>SNLEQIDAELVLSIEKLQEIQDDLEKINEKASDEVLEVEQKYNVIRKPVYDKRNEVIQSIPGFWMTAFLSHPALGDLLTEEDQKIFKYLNSLEVEDAKDVKSGYSITFHFTSNPFFEDAKLTKTFTFLEEGTTKITATPIKWKEGKGLPNGVNHDDKKGNKRALPEES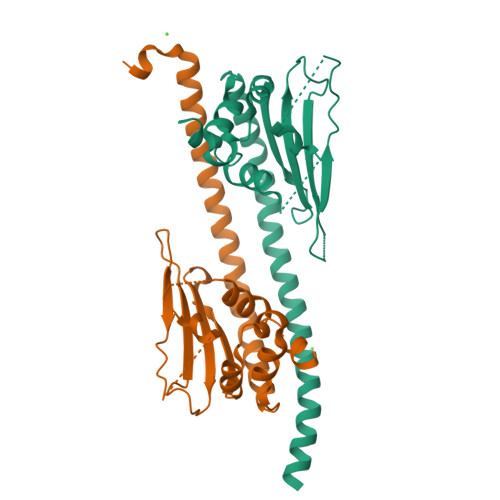FFTWFTDAQHKEDAGDEIHDEVADIIKEDLWSNPLTYFNN[2x]>[8x]SNAMFIQNEHVGDRSRMEDWRIRGYDPLAPPDLLQHEFPLSDKNKDIILKGREDTCNILNGKDDRLIVVIGPCSIHDPEAALDYADRLHKLSEKHKGELHIVMRAYL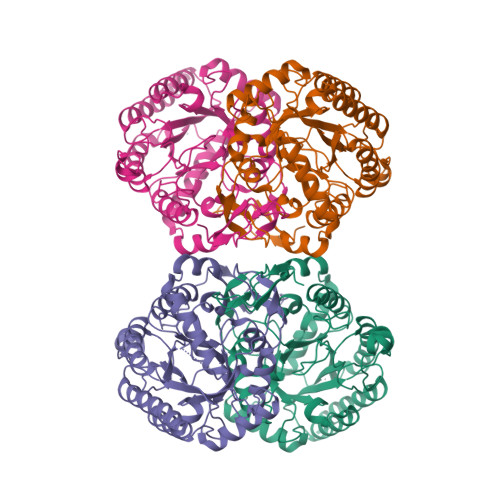EKPRTTVGWKGLINDPDIDGSFQINKGLRIARKMFVQLTEKLPIAGEMLDTISPQFLSDLFSVGAIGARTTESQLHRELASGLSFPVGFKNGTDGTLGVAIDALRAASHPHHFLSVTKPGIVSIVGTEGNQDCFVILRGGKQGTNYDAKSVKETKEALAKAKVVDPENPKPRIMVDCSHGNSNKNHKNQPLVAADVAKQISEGEDQICGLMIESNINEGRQDVPPADKGGKEALKYGCSITDACIGIDDTESVLETLAQAIKARRGLKS> GHMFQCNVPLGMESGRIANEQISASSTYSDGRWTPQQSRLHGDD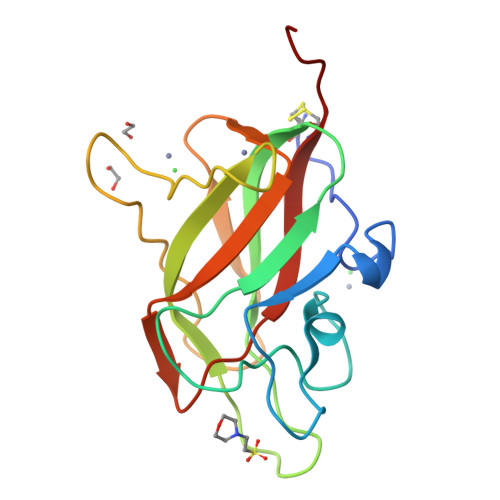NGWTPNLDSNKEYLQVDLRFLTMLTAIATQGAISRETQNGYYVKSYKLEVSTNGEDWMVYRHGKNHKVFQANNDATEVVLNKLHAPLLTRFVRIRPQTWHSGIALRLELFGCRVTSGS>[3x]MEQQPAAAEPEVPAGLGLTA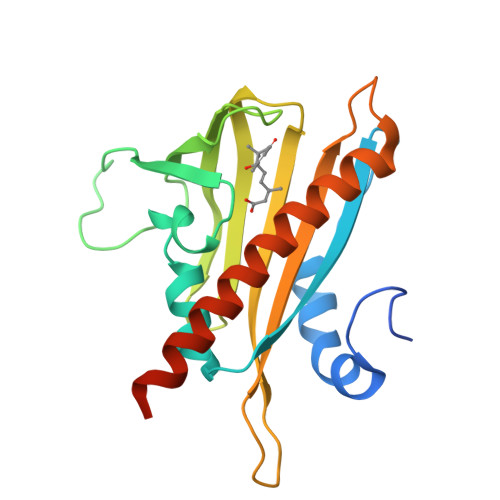AEYAELQPTVEAYHRYAVGPGQCSSLVAQRIEAPAAAVWAIVRRFDCPQVYKHFIRSCALRPDPDAGDELRPGRLREVSVISGLPASTSTERLDLLDDARRAFGFTITGGEHRLANYRSVTTVSELAPAAPAKICTVVLESYVVDVPEGNSEEDTRLFADTVVRLNLQKLKSLAEANATSAAAQATPPPQAE>GHMTASPRAPHQEHVLGEPTLEGLAHYIREKNVRRILVLVGAGASVAAGIPDFRSPDTGIYANLGKYNLEDPTDAFSLTLLREKPEIFYSIARELNLWPGHFQPTAVHHFIRLLQDEGRLLRCCTQNIDGLEKAAGVSPELLVEAHGSFAAAACIECHTPFSIEQNYLEAMSGTVSRCSTCGGIVKPNVVFFGENLPDAFFDALHHDAPIAELVIIIGTSMQVHPFALLPCVVPKSVPRVVMNRERVGGLLFRFASTSSSSDGYGQYGDYHAHPDVCRDVLFRGDCQENVVTL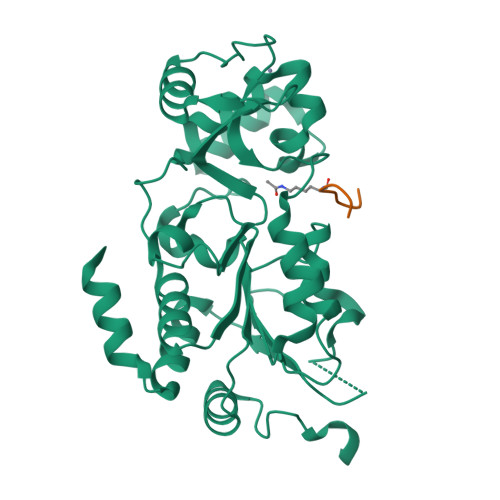AEYLGLSEALAKRMRLSDAAPATAQRAPNET[2x];>[2x]KKGQSTSRHKKLMFKTEG>[5x]MTITYTSQVANARLGSFSRLLLCWRGSIYKLLY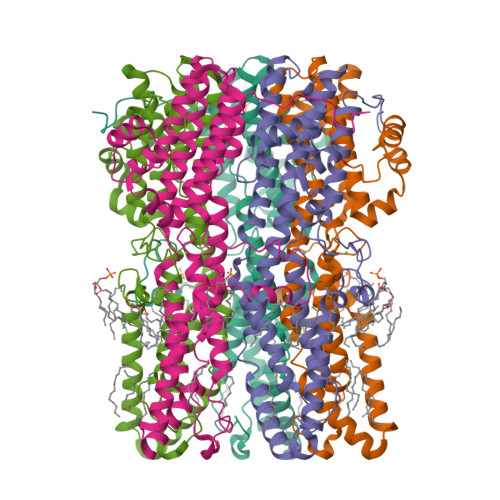GEFLIFLLCYYIIRFIYRLALTEEQQLMFEKLTLYCDSYIQLIPISFVLGFYVTLVVTRWWNQYENLPWPDRLMSLVSGFVEGKDEQGRLLRRTLIRYANLGNVLILRSVSTAVYKRFPSAQHLVQAGFMTPAEHKQLEKLSLPHNMFWVPWVWFANLSMKAWLGGRIRDPILLQSLLNEMNTLRTQCGHLYAYDWISIPLVYTQVVTVAVYSFFLTCLVGRQFLNPAKAYPGHELDLVVPVFTFLQFFFYVGWLKVAEQLINPFGEDDDDFETNWIVDRNLQVSLLAVDEMHQDLPRMEPDMYWNKPEPQP> APYNGNPFEGVQLWANNYYRSEVHTLAIPQITDPALRAAASAVAEVPSFQWLDRNVTVDTLLVQTLSEIREANQAGANPQYAAQIVVYDLPDRDCAAAASNGEWAIA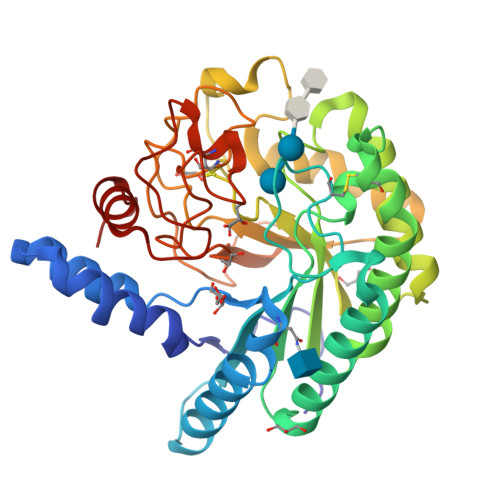NNGVNNYKAYINRIREILISFSDVRTILVIEPDSLANMVTNMNVPKCSGAASTYRELTIYALKQLDLPHVAMYMDAGHAGWLGWPANIQPAAELFAKIYEDAGKPRAVRGLATNVANYNAWSVSSPPPYTSPNPNYDEKHYIEAFRPLLEARGFPAQFIVDQGRSGKQPTGQKEWGHWCNAIGTGFGMRPTANTGHQYVDAFVWVKPGGECNGTSDTTAARYDYHCGLEDALKPAPEAGQWFNEYFIQLLRNANPPF>MFEIKKICCIGAGYVGGPTCSVIAHMCPEIRVTVVDVNESRINAWNSPTLPIYEPGLKEVVESCRGKNLFFSTNIDDAIKEADLVFISVNTPTKTYGMGKGRALDLKYIEACARRIVQNSNGYKIVTEKSTVPVRAAESIRRIFDANTKPNLNLQVLSNPEFLAEGTAIKDLKNPDRVLIGGDETPEGQRAVQALCAVYEHWVPREKILTTNTWSSELSKLAANAFLAQRISSINSISALCEATGADVEEVATAIGMDQRIGNKFLKASVGFGGSCFQKDVLNLVYLCEALNLPEVARYWQQVIDMNDYQRRRFASRIIDSLFNTVTDKKIAILGFAFKKDTGDTRESSSIYISKYLMDEGAHLHIYDPKVPREQIVVDLSHPGVSEDDQVSRLVTISKDPYEACDGAHAVV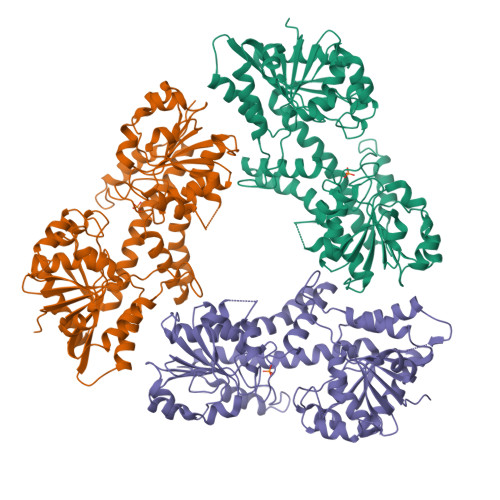ICTEWDMFKELDYERIHKKMLKPAFIFDGRRVLDGLHNELQTIGFQIETIGKKVSSKRIPYAPSGEIPKFSLQDPPNKKPKV[3x]>[6x]SGSGSTAEPDLKTALKAVIPAKRELFKQVKERSDEVIGEVKVANVIGGMRGLKSMLWEGSVLDPEEGIRFHGKTIKDCQKELPKGTSGTEMLPEAMFWLLLTGQVPSTNQVRAFSRELAEQSH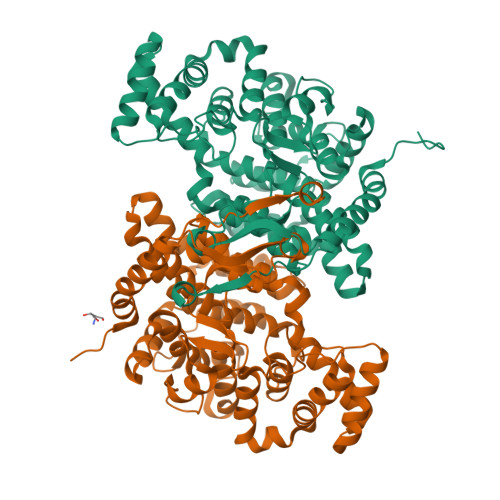LPQHILDLIKSFPRSMHPMTQLSIAVAALNTESKFAKAYEKGLSKADYWEPTFDDSISLLAKIPRVAALVFRPDEVDQVGTQALDASQDWSYNFAELLGKGGKENQDFHDLLRLYLALHGDHEGGNVSAHATHLVGSALSDPFLSYSAGLLGLAGPLHALAAQEVLRWILAMQDKIGTKFTDDDVRNYLWDTLKSGRVVPGYGHGVLRKPDPRFQALMDFAATRPDVLANPVFQLVKKNSEIAPAVLTEHGKTKNPHPNVDAASGVLFYHYGFQQPLYYTVTFGVSRALGPLVQLIWDRALGLPIERPKSINLLGLKK> NKITPNLAEFAFSLYRQLAHQSNSTNIFFSPVSIATAFAMLSLGTKADTHDEILEGLNFNLTEIPEAQIHEGFQELLRTLNQPDSQLQLTTGNGLFLSEGLKLVDKFLEDVKKLYHSEAFTVNF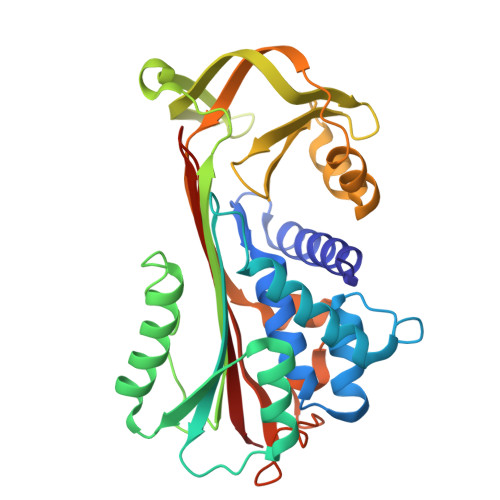GDTEEAKKQINDYVEKGTQGKIVDLVKELDRDTVFALVNYIFFKGKWERPFEVKDTEEEDFHVDQVTTVKVPMMKRLGMFNIQHCKKLSSWVLLMKYLGNATAIFFLPDEGKLQHLENELTHDIITKFLENEDRRSASLHLPKLSITGTYDLKSVLGQLGITKVFSNGADLSGVTEEAPLKLSKAVHKAVLTIDEKGTEAAGAMFLEAIPM~{N}-[4-(4-chloranylphenoxy)phenyl]-7~{H}-pyrrolo[2,3-d]pyrimidin-4-amine 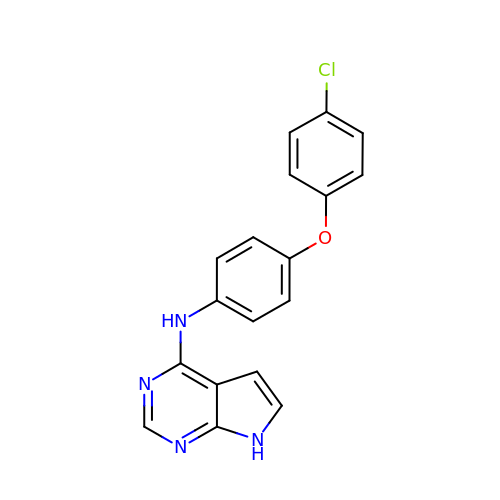| C18 H13 Cl N4 O | RWRSKMSFZCQDMQ-UHFFFAOYSA-N Methanobactins (Mbns) are a family of copper-binding peptides involved in copper uptake by methanotrophs, and are potential therapeutic agents for treating diseases characterized by disordered copper accumulation. Mbns are produced via modification of MbnA precursor peptides at cysteine residues catalyzed by the core biosynthetic machinery containing MbnB, an iron-dependent enzyme, and MbnC. Here, we present crystal structures of MbnABC complexes from two distinct species, revealing that the leader peptide of the substrate MbnA binds MbnC for recruitment of the MbnBC holoenzyme, while the core peptide of MbnA resides in the catalytic cavity created by the MbnB–MbnC interaction which harbors a unique tri-iron cluster. In both structures, the interactions between MbnA, MbnB and MbnC result in the formation of a 1:1:1 tertiary complex, and the overall structures of VcMbnABC and RrMbnABC are nearly identical.

To understand the mechanism of how MbnBCs catalyze modification of MbnAs, we finally solved the crystal structures of VcMbnABC and RrMbnABC at resolutions of 2.2 Å and 2.7 Å, respectively. Similar to MtMbnABC,17 the three components of RrMbnABC formed a stable complex when co-expressed in Escherichia coli. High-resolution mass spectrometry (MS) indicated that the absorption resulted from modifications on either Cys21 or Cys25. In contrast to VcMbnA, the C-terminal half of the RrMbnA LP (residues 15–20) forms a short kink, which interacts with the surface loop region of RrMbnB. Formation of the kink allows the second cysteine residue (Cys25) to coordinate to one of the iron ions in the catalytic cavity of RrMbnBC. The divalent ion (Fe1) coordinates to VcMbnAC18 in VcMbnABC and to RrMbnAC25 in RrMbnABC, providing direct evidence for cysteine modifications of MbnA by MbnBC. RrMbnBC can modify either Cys21 or Cys25 of RrMbnA as indicated by MS data, but only Cys25 was found to coordinate to Fe1 in the crystal structure of RrMbnABC. This may be a more energetically favorable binding mode for RrMbnA to interact with the catalytic site of RrMbnBC and could therefore be more readily captured by crystallography. Consistent with this hypothesis, our enzymatic assays showed that RrMbnBC was active in modifying MbnAs from Groups I–V. VcMbnB Asp240 and the equivalent in RrMbnB, Asp242, are conserved among MbnBs and are located adjacent to the apex of the curved portion of MbnA.

>MKIVIVKKVEIQVAGRTGMRCASSCGAKS[2x];> MRIGFNFTLGETLPLVRQLAQEGAIDYCELLIDNFMQVPPQELAEAFDVPVGFHIMFSRFIESDEEQLRDFAARLRPYIEALRPLYVSDHIAYFSHQGRALYHLGEIDYAADYERVRARAALWQSLLGQTIHFENYPSIVDGGHAAPAFFQRLARDTGAGVLFDVSNAVCAWRNDGPEVAAWRGVMAGASHFHVGGYAGAFIDEGVTVDTHDRALAQDTLDSLRRHRDVLDKPGATITYERDENIDIDGVRADLLALRAIFPR;>[2x]MNAPTTAAAGAAPGRQVKDSELLARLADPAARGDFPPGCRAHVRIDISIRAYWHTLFDICPGLLDIADPDGMAIFAPFMDWARRENLTMGWSFYIWVGRWLAQSPWRERLDEELTQALLSASAARWAVLDRSADVGVVLGRRGSDDWIIGWKPNTLAAGRRVELVSLDGQLPRPAEDVGVFHLAGYELDSFPGWLALPR;> MRIGFNFTLGETLPLVRQLAQEGAIDYCELLIDNFMQVPPQELAEAFDVPVGFHIMFSRFIESDEEQLRDFAARLRPYIEALRPLYVSDHIAYFSHQGRALYHLGEIDYAADYERVRARAALWQSLLGQTIHFENYPSIVDGGHAAPAFFQRLARDTGAGVLFDVSNAVCAWRNDGPEVAAWRGVMAGASHFHVGGYAGAFIDEGVTVDTHDRALAQDTLDSLRRHRDVLDKPGATITYERDENIDIDGVRADLLALRAIFPRG>[2x]MQYATLELN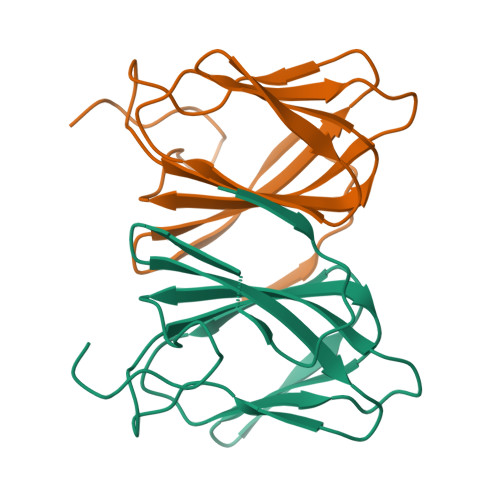NAFKVLFSLRQVQAAEMVIAPGDREGGPDNRHRGADQWLFVVDGAGEAIVDGHTQALQAGSLIAIERGQAHEIRNTGDTPLKTVNFYHPPAYDAQGEPLPAGEG>[4x]GATESGKRMDCPALPPGW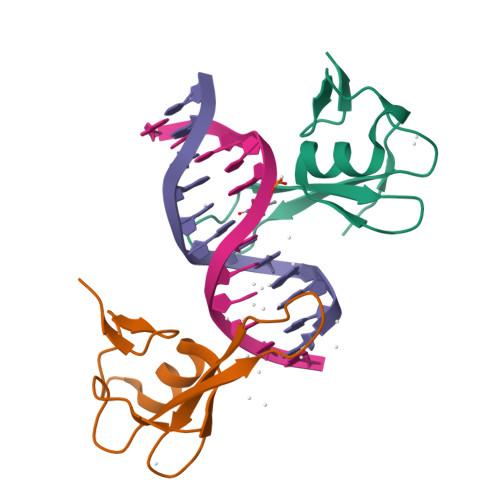KKEEVIRKSGLSAGKSDVYYFSPSGKKFRSKPQLARYLGNTVDLSSFDFRTGKMMPSKLQK>[2x]GSHMLIYQAIKLIAQAIKVIAEAIKAIAEGDKERAKEAAEKARELYEKALELYKEAKKEGDLIAAAIALIAAAIAVIALAIAAIAAGDKELAKEAAELAKEIYKLAEKLYKEAKKKGDLIAAAIALIAAAIAVIALAIAAIAAGDKELAKEAAKLAKEVYKEAEELYREARKKGDLIAAAIALIAAAIAVIALAIAAIAAGDKELAKKAAELAEKVYKEALKVYKEARKKGDLIAAAIALIAAAIAVIALAIAAIAAGDKELAKKAAELAKKVLELAREIAKEARKKGDLIAAAIALIAAAIAVIALAIAAIAAGDKEEAKEAYELAKEVYKEALEIAKEARKKGDYIAAAIAAIAAAIAVIAAAIAAIAAGDKEEAKEAYKLAKEAKEKAKEIAKEAKKAGDKIAAAIAEIAQAIAEIAQAIAEIALK

Here we describe efficient routes starting from validated parallel and antiparallel peptide assemblies to design two families of α-helical barrel proteins with central channels that bind small molecules. Computational designs are seeded by the sequences and structures of defined de novo oligomeric barrel-forming peptides, and adjacent helices are connected by loop building. For targets with antiparallel helices, short loops are sufficient. However, targets with parallel helices require longer connectors; namely, an outer layer of helix–turn–helix–turn–helix motifs that are packed onto the barrels.

Encouraged by the successful design of sc-apCC-6 and sc-CC-7, we extended the seeded design approaches to target α-helical barrel proteins with five, six and eight central helices. By contrast, the six- and eight-helix-based targets bound dye, consistent with accessible cavities, which were confirmed by SEC-SAXS and X-ray crystal structures solved using molecular replacement. Together, these additional designs delivered the de novo proteins sc-CC-5, sc-CC-6 and sc-CC-8. For the parallel targets, the experimental structures show minor fraying at the C termini of the inner helices compared with the seeds and models, which appears to improve the packing of the external three-helix bundles. However, the symmetry of the central parallel helices is maintained. The backbone RMSD values for the repeating helix–turn–helix–turn–helix motifs are ≤0.5 Å, which is expected given the low sequence variation in the loops and the hydrophobic cores of these buttressing helices. The parallel designs all showed some similarity with natural and designed helical solenoid proteins.> VSDLPPSVDWRQKGAVTGVKDQGKCGSCWAFSTVVSVEGINAIRTGSLVSLSEQELIDCDTADNDGCQGGLMDNAFEYIKNNGGLITEAAYPYRAARGTCNVARAAQNSPVVVHIDGHQDVPANSEEDLARAVANQPVSVAVEASGKAFMFYSEGVFTGECGTELDHGVAVVGYGVAEDGKAYWTVKNSWGPSWGEQGYIRVEKDSGASGGLCGIAMEASY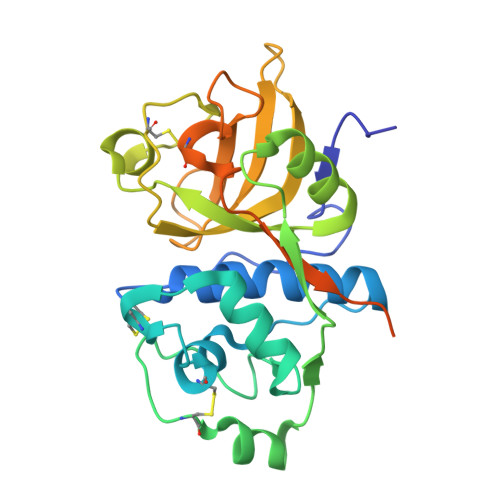PVKTYSKPKPTPRRALGARESLNSSSVDKLAAALEHHHHHH>KALPEGPGEKRADLIEIGAMERFGKLDLPKVAFRHDQHTTAVTGMGKDCAACHKSKDGKMSLKFMRLDDNSAAELKEIYHANCIGCHTDLAKAGKKTGPQDGECRSCHNPKPSAASSWKEIGFDKSLHYRHVASKAIKPVGDPQKNCGACHHVYDEASKKLVWGKNKEDSCRACHGEKPVDKRPALDTAAHTACISCHMDVAKTKAET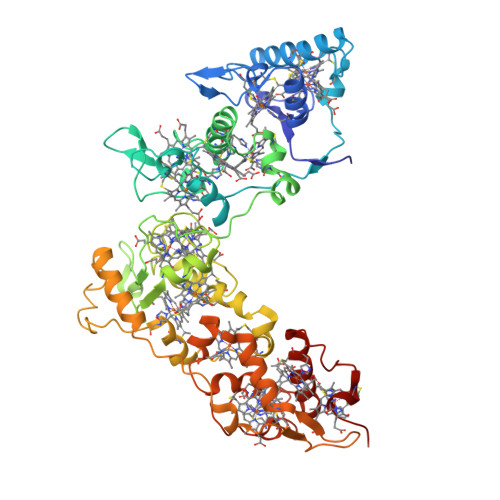GPVNCAGCHAPEAQAKFKVVREVPRLDRGQPDAALILPVPGKDAPREMKGTMKPVAFDHKAHEAKANDCRTCHHVRIDTCTACHTVNGTADSKFVQLEKAMHQPDSMRSCVGCHNTRVQQPTCAGCHGFIKPTKSDAQCGVCHVAAPGFDAKQVEAGALLNLKAEQRSQVAASMLSARPQPKGTFDLNDIPEKVVIGSIAKEYQPSEFPHRKIVKTLIAGIGEDKLAATFHIEKGTLCQGCHHNSPASLTPPKCASCHGKPFDADRGDRPGLKAAYHQQCMGCHDRMKIEKPANTACVDCHKERAK[4x]>[12x]MLRMNPGLGSSISVHPSELSISLFEILQGKYSYVRGQTLHCSLRNPGVFFRQLFIHLYKNALANCSYDHVLSDWRTYESSAKTRWPEKEAQWGSYRRSTFDSWAQ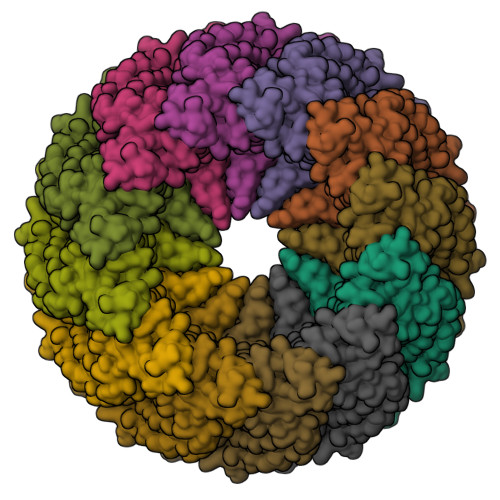TMRMTLDHLLLNAINRVLYAKTQLSYERYVDWVVTVGMVPVVKHTPDHKLVNSIQEQLMKDCQRLASGEKTIGRILTSVTQEISNLVSSLSALYIPGYSEVSIDYDCVKNTFVGLYKQKRVHVEVITMPAILAGRVIFDSPIQRMYTSIMSCHRTAEHAKLCQLLNTAPTKALVGSACNNVYKDIMTHLEQASQRTDPKRELLNLLMKLAENKTVSGVTDVVEDFVTDVSQNIVDKNKLFGTGQETTTQGLRRQVSNSVFKCLTNQINEQFDTITQLEKERELCMKRLKCIETQLSHQQPGDAKGPGSVNLLTANTFQSLGRLQDPSLQLTSSHIPSGSAVLNSFFSSYIPPVRESMKDLTNLWESEMFQTYKLAPVVDNQGQRLSVTYSQDTISILLGPFTYVIADLLQMELISHSFVSSSLQDIAAYLYQTSRLFVYITDVGQKYCLVTPPFENVPGKGPGETDWSANEYSCPEDSRVRRGLSRIPPPCGAPPCPGSA>SMEDPDQLYTTLKNLLAQIKSHPSAWPFMEPVKKSEAPDYYEVIRFPIDLKTMTERLRSRYYVTRKLFVADLQRVIANCREYNPPDSEYCRCASALEKFF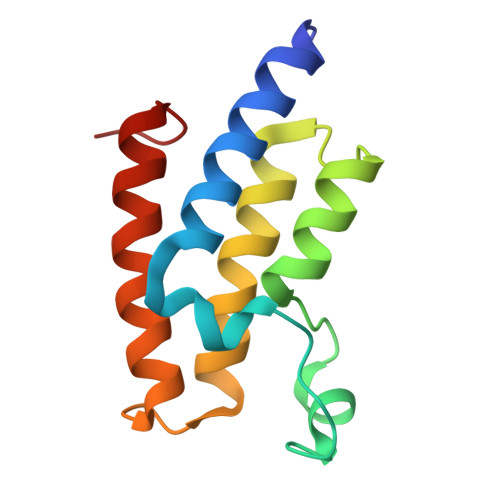YFKLKEGGLIDK[2x]>SMRIVALDGYTLNPGDISWAPIEELGELVVHPRTPSDKIIERAAGAHVVLTNKVP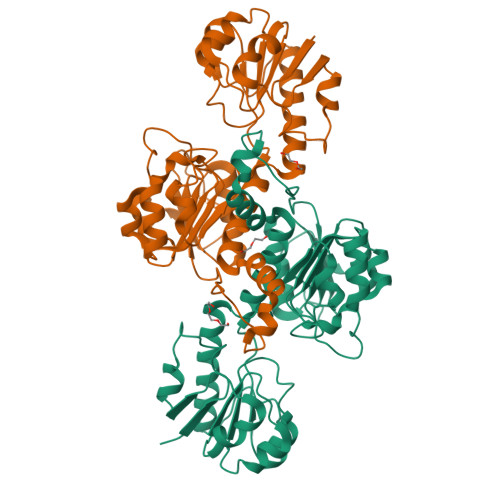LDMSALQALPGLRFVSVLATGYDKVDVAAAGVLGIPVSNVPGYGTDSVAQHVFALLLELCRRTALHDHRIRAGAWTQSPDWCFWDSTQEELTGKTMGIVGFGNTGRRVGRIANALGMNVIAYAPRSRFDPDYRPFEHVGLDELFTSADVVSLHCPLTPETEGLVDARRLASMRPGSYLINTARGPLLDERAVAEALDSGRLAGAGLDVLSQEPPAADNPLLSAKNCLITPHLAWASRTARRTLMDSTAANIRSFIEGTPVNVVNAAHLRTKG[2x]>[4x]SNIDHSKNNIIEEFDKLSDDFSNDINATKQTIKD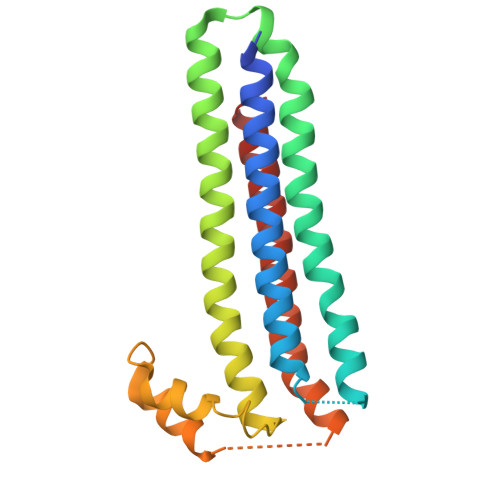LFLDIEASFEDTSDDVVKLLSKYSFVPEEKLNIIDGILRSFIENNKTHVINSSNAYIYIQKEKIKNVCNFILKKLNSLIQINELNKSHIILKYGKGEAKKGVLESIKNNDDISKNLKSELLKYENVNNQNIRVSELINFITPIYDDFIKNLTDLINDLQIKLKNISK>[2x]MNLPTAQEVQGLMARXIELVDVGDIEAIVQMYADDATVENPFGQPPIHGREQIAAFYRQGLGGGKVRACLTGPVRASHNGCGAMPFRV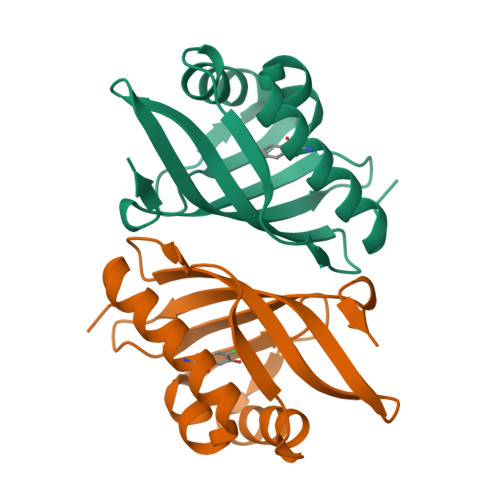EMVWNGQPCALDVIDVMRFDEHGRIQTMQAYWSEVNLSVREPQLVPR> ALKTLNLGSCVIATN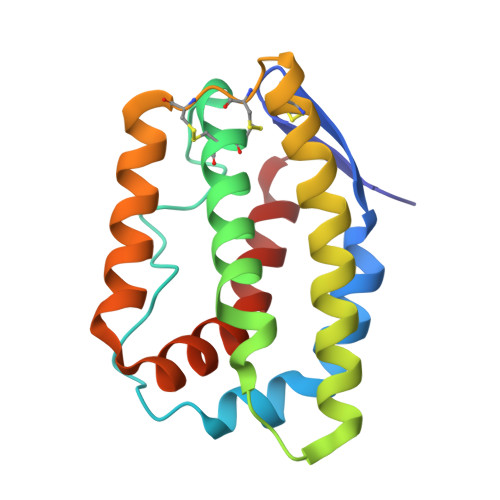LQEIRNGFSEIRGSVQAKDGNIDIRILRRTESLQDTKPANRCCLLRHLLRLYLDRVFKNYQTPDHYTLRKISSLANSFLTIKKDLRLCHAHMTCHCGEEAMKKYSQILSHFEKLEPQAAVVKALGELDILLQWMEETE>GSGMQKLTILGATGSIGASTLKVIEQNPDKFSVVALAADSNVEKMQQLCQRWQPEYAVMANKEAALRLKMALAVLAPNTQVLGGQEALCYVATLEQVDSVMAAIVGAAGLVPTMAAVKAGKRILLANKEALVMSGQLFIDEVEKSGAQLLPVDSEHNAIFQCLPQTVQGNLGRCDLASQGVSHILLTGSGGPFRYTDVAELEAVTPEQAIAHPNWSMGPKISVDSATMMNKGLEYIEAKWLFNASRDQLKVIIHPQSVIHSMVQYLDGSV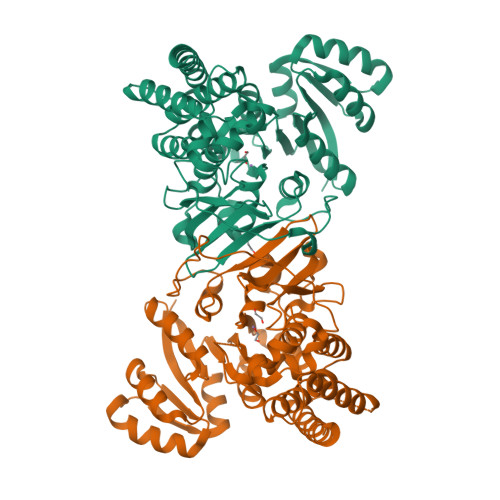LAQMGEPDMATPIALTLSYPERVKAGVKPLDFTQVGELTFLQPDFERYPCLALAIEACYLGQHATTTLNAANEVAVAAFLARQIKFTDIARVNDSVLNQVCKQSLASGLDSLESLLELDRMARTLADEVVRERAQ[2x]> MSRSRPELGDWSSPAELAELQRSQLPRVLAQALRSPFYAARYRGTTPPRTADDFAGVEVTAKQDLRDQYPFGMLAVGREHLATYHESSGTAGEPTASYYTEEDWTDLAERFARKWTGIHPSDTFLVRTPYGLVITGHLAQAAGRLRGATVVPGDARSLATPLSRMVRVLKTLDVTLTWCNPTEITMLAAAAKAAGLRPDQDFPHLRAMFTAAEPLTEVRRRRLSEIWGGIPVVEEYGSTETGTIAGQCPEGRMHLWADRAIFEVYDPRTGTLSEAGRGQMVVTPLYRDAMPLLRYNLADDVEVSTDPCGCGWLLPTVTVLGRAGTGHRIGPATVTQQRLEELVFSLPAAYEVMFWRAKAHPDVLELEFEAPEPVRQRAVKELGAALDRELGVPHRITGLAPGTLVPAEALTAQRDILKARYLFAEDEDWDKAVMYF;> AMSRSRPELGDWSSPAELAELQRSQLPRVLAQALRSPFYAARYRGTTPPRTADDFAGVEVTAK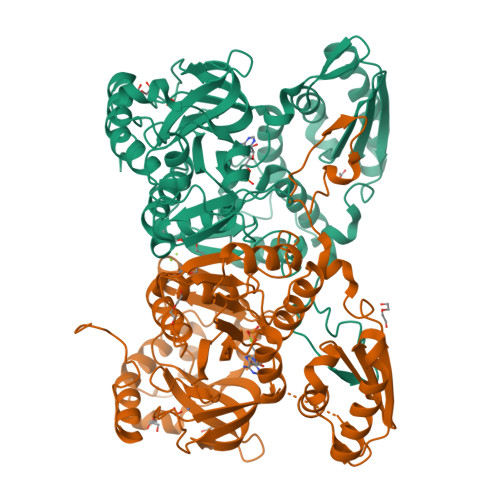QDLRDQYPFGMLAVGREHLATYHESSGTAGEPTASYYTEEDWTDLAERFARKWTGIHPSDTFLVRTPYGLVITGHLAQAAGRLRGATVVPGDARSLATPLSRMVRVLKTLDVTLTWCNPTEITMLAAAAKAAGLRPDQDFPHLRAMFTAAEPLTEVRRRRLSEIWGGIPVVEEYGSTETGTIAGQCPEGRMHLWADRAIFEVYDPRTGTLSEAGRGQMVVTPLYRDAMPLLRYNLADDVEVSTDPCGCGWLLPTVTVLGRAGTGHRIGPATVTQQRLEELVFSLPAAYEVMFWRAKAHPDVLELEFEAPEPVRQRAVKELGAALDRELGVPHRITGLAPGTLVPAEALTAQRDILKARYLFAEDEDWDKAVMYF> GPLGSETITVPTPIKQIFSDDAFAETIKDNLKKKSVTDAVTQNELNSIDQIIANNSDIKSVQGIQYLPNVTKLFLNGNKLTDIKPLANLKNLGWLFLDENKVKDLSSLKDLKKLKSLSLEHNGISDINGLVHLPQLESLYLGNNKITDITVLSRLTKLDTLSLEDNQISDIVPLAGLTKLQNLYLSKNHISDLRALAGLKNLDVLELFSQECLNKPINHQSNLVVPNTVKNTDGSLVTPEIISDDGDYEKPNVKWHLPEFTNEVSFIFYQPVTIGKAKARFHGRVTQPLKEVYTVSYD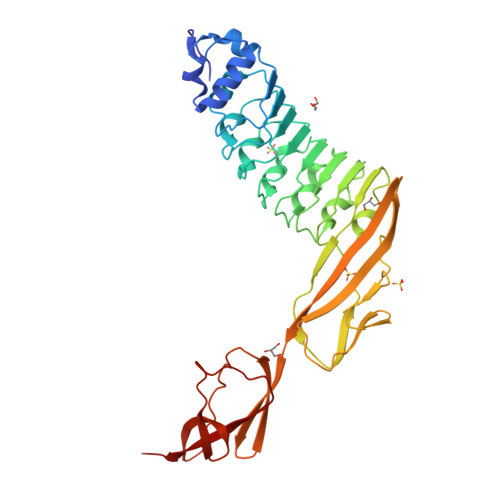VDGEVIKTKVEAGTRITAPKPPTKQGYVFKGWYTEKNGGHEWNFNTDYMSGNDFTLYAVFKAET>[5x]TP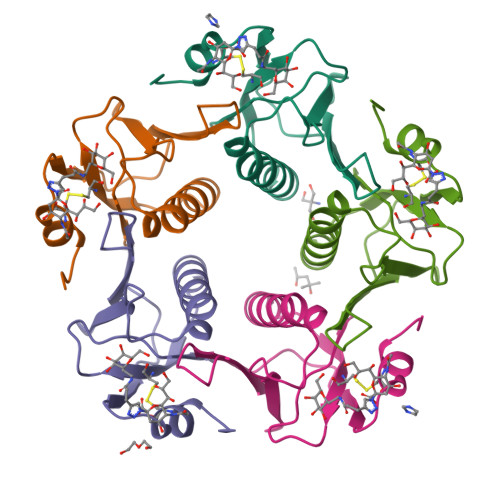QNITDLCAEYHNTQIYTLNDKIFSYTESLAGKREMAIITFKNGAIFQVEVPGSQHIDSQKKAIERMKDTLRIAYLTEAKVEKLCVWNNKTPHAIAAISMAN>HHHHHHENLYFQGSGSSPRSGVLLRGCPTHCHCEPDGRMLLRVDCSDLGLSELPSNLSVFTSYLDLSMNNISQLLPNPLPSLRFLEELRLAGNALTYIPKGAFTGLYSLKVLMLQNNQLRHVPTEALQNLRSLQSLRLDANHISYVPPSCFSGLHSLRHLWLDDNALTEIPVQAFRSLSALQAMTLALNKIHHIPDYAFGNLSSLVVLHLHNNRIHSLGKKCFDGLHSLETLDLNYNNLDEFPTAIRTLSNLKELGFHSNNIRSIPEKAFVGNPSLITIHFYDNPIQFVGRSAFQHLPELRTLTLNGASQITEFPDLTGTANLESLTLTGAQISSLPQTVCNQLPNLQVLDLSYNLLEDLPSFSVCQKLQKIDLRHNEIYEIKVDTFQQLLSLRSLNLAWNKIAIIHPNAFSTLPSLIKLDLSSNLLSSFPITGLHGLTHLKLTGNHALQSLISSENFPELKVIEMPYAYQCCAFGVCENAYKISNQWNKGDNSSMDDLHKKDAGMFQAQDERDLEDFLLDFEEDLKALHSVQCSPAAA[4x];>GSRISAEGSQACAK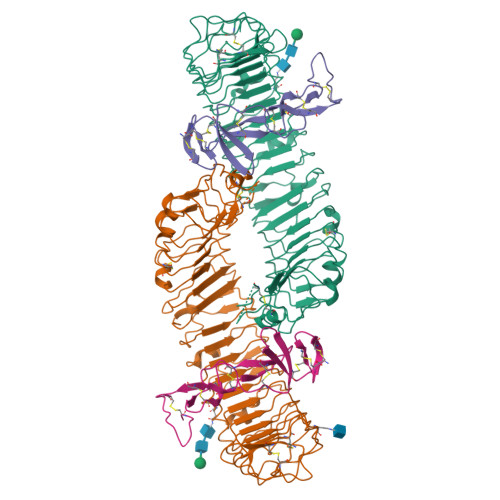GCELCSEVNGCLKCSPKLFILLERNDIRQVGVCLPSCPPGYFDARNPDMNKCIKCKIEHCEACFSHNFCTKCKEGLYLHKGRCYPACPEGSSAANGTMECSSPAAAHHHHHH[4x]> MELIKGQALFLELDKKDFLSLKNNDKNIPTFAHPKNQEKILAIFSLPYKNPPQNTKLIAFYKDKKEEIFIKTLEGNYKSEKLQVENKKIFPPKTIQERIAKELKEANAIYSSYTPKALFNGAFNIPLNSFITSDFGKARTFNEKVASYHSGTDFRAATGTPIYAANSGVVKIAKDRYFAGNSVVIDHGFGIY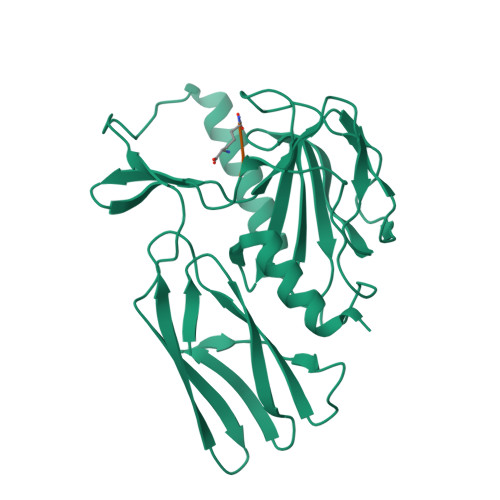SQYYHLSKIDVKVGQKIKKGELIGLSGASGRVSGPALHFGILAGGKQVDPLDFVSKFNAIFQL>MSLDEDKTNDSAFHARLIAEVLEAYPDKARKRRQKHLNVAGQAEAEAQDAGEEGVMLSECDVKSNVKSVPGVMTIRGCAYAGSKGVVWGPVKDMVHISHGPVGCGQYSWSQRRNYYIGNTGVDSFVTMQFTSDFQEKDIVFGGDKKLEKIIDEIDELFPLAKGISVQSECPIGLIGDDIEAVSRKKKKEIGKTIVPVRCEGFRGVSQSLGHHIANDAIRDWVFDGEDKHAAFETTPYDVNVIGDYNIGGDAWSSRILLEEMGLRVVGNWSGDATLAEIERAPKAKLNLIHCYRSMNYICRHMEEKYNIPWTEYNFFGPSQIAASLRKIAALFDEKIQEGAERVIAKYQPLVDAVIEKFRPRLAGKKVMLYVGGLRPRHVVNAYNDLGMEIVGTGYEFGHNDDYQRTGHYVREGTLIYDDVTGYELEKFIEGIRPDLVGSGIKEKYPVQKMGIPFRQMHSWDYSGPYHGYDGFAIFARDMDLAINNPVWSMFKAPWKNAA[2x];>[2x]MPQNVDKILDHAPLFREPEYQEMLAGKAKLENMPPADKVVEIADWTKSWEYREKNFARESLSVNPAKACQPLGAVFVASGFERTMSFVHGSQGCVAYYRSHLSRHFKEPSSAVSSSMTEDAAVFGGLNNMVDGLANTYKLYDPKMIAVSTTCMAEVIGDDLHAFIQTAKGKGSVPEEFDVPFAHTPAFVGSHVTGYDNMLKGILEHFWKGRTPVPNRSVNIIPGFDGFAVGNNRELKRILGMMGVQYTILSDVSDQFDTPSDGEYRMYDGGTKIEAARDAVNADYTISLQEYCTPKTLEYCQSFGQKTASFHYPLGIGATDDLLQKLSEISGKPVPQELEMERGRLVDALADSQAYLHGKTYAIYGDPDFVYGMARFILETGGEPKHCLATNGSKAWEAQMQELFDSSPFGVGCKAWGGKDLWHMRSLLATEKVDLLIGNSYGKYLERDTDTPLIRLMFPIFDRHHHHRFPVWGYQGALRVLVTLLDK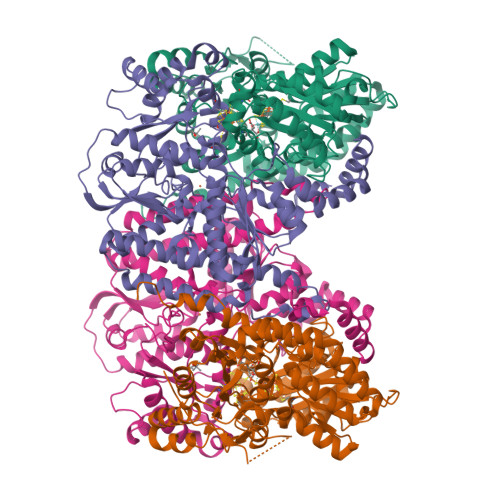IFDKLDDDTIQAGVTDYSFDLTR>[2x]MNTTPVHALTDIDGGIAVDPAPRLAGPPVFGGPGNDAFDLAPVRSTGREMLRFDFPGVSIGAAHYEEGPTGATVIHIPAGARTAVDA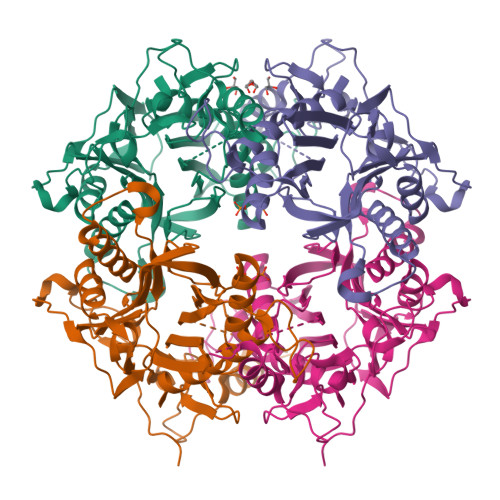RGGAVGLSGGYDFNHAICLAGGAGYGLEAGAGVSVALLERLEHRTGFAELQLVSSAVIYDFSARSTAVYPDKALGRAALEFAVPGEFPQGRAGAGMSASAGKVDWDRTEITGQGAAFRRLGDVRILAVVVPNPVGVIVDRAGTVVRGNYDAQTGVRRHPVFDYQEAFAEQVPPVTEAGNTTISAIVTNVRMSPVELNQFAKQVHSSMHRGIQPFHTDMDGDTLFAVTTDEIDLPTTPGSSRGRLSVNATALGAIASEVMWDAVLEAGK N-{[(3S,5S)-5-(1,3-THIAZOLIDIN-3-YLCARBONYL)PYRROLIDIN-3-YL]METHYL}-1,3-THIAZOLE-4-CARBOXAMIDE 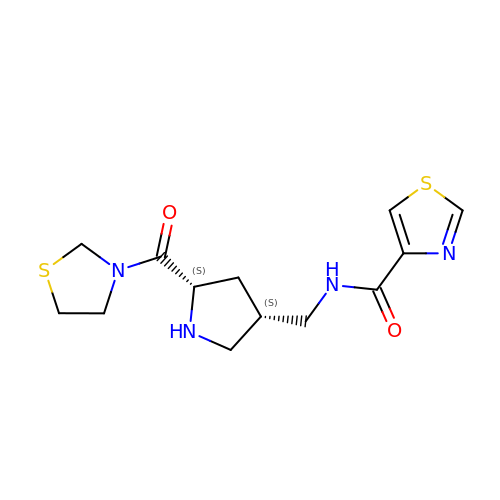| C13 H18 N4 O2 S2 | KFQMVMSMRNCTET-UWVGGRQHSA-N>[2x]MLSPIRTTFHNSVNIVQSSPSQTVSFAGKEYELKVIDEKTPILFQWFEPNPER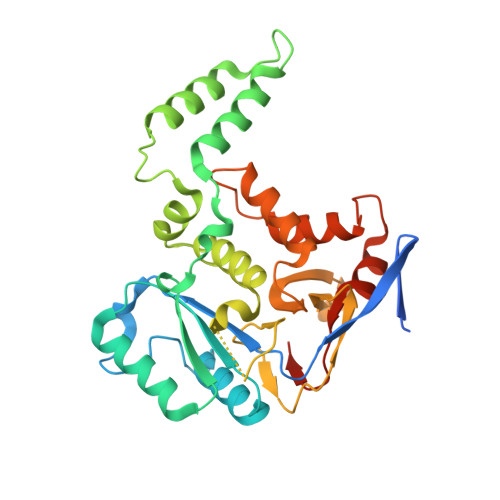YKKDEVPIVNTKQHPYLDNVTNAARIESDRMIGIFVDGDFSVNQKTAFSKLERDFENVMIIYREDVDFSMYDRKLSDIYHDIICEQRLRTEDKRDEYLLNLLEKELREISKAQDSLISMYAKKRNHAWFDFFRNLALLKAGEIFRSTYNTKNHGISFGEGCIYLDMDMILTGKLGTIYAPDGISMHVDRRNDSVNIENSAIIVNRSNHPALLEGLSFMHSKVDAHPYYDGLGKGVKKYFNFTPLHNYNHFCDFIEFNHPNIIMNTSQYTCSSW> MGSSHHHHHHMAYTNTPHNWGIPRPKNETVPDAGKLYTDLLQKNGGFYLGDTKKKDIYLTFDNGYENGYTGKILDVLKEKKVPATFFVTGHYIKTQKDLLLRMKDEGHIIGNHSWSHPDFTAVNDEK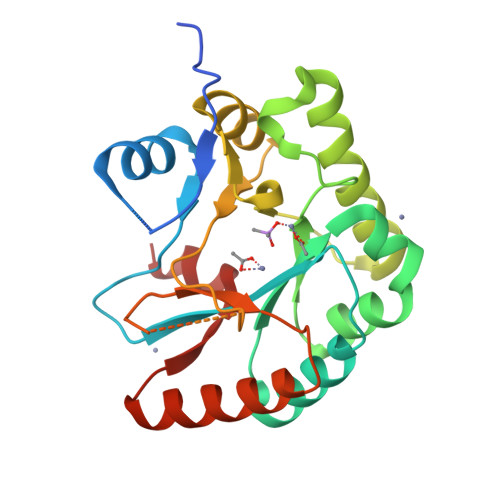LREELTSVTEEIKKVTGQKEVKYVRPPRGVFSERTLALTKEMGYYNVFWSLAFLDWKVDEQRGWQYAHNNVMTMIHPGSILLLHAISKDNAEALAKIIDDLREKGYHFKSLDDLVKSNQP> MWHYTSINNDTRVALDPKPNQIRTITKPNTVPQLGTDYLYTFNSQRRSHTLRLLGPFQYFNFSETDRGHPLFRLPLKYPSKAIPADELIDNLHSWMRSVHLLHVRSEDNTLRYNWMLGVYARSTNYTTPVGQLVVNAPAILNYSNPQDAFNSVFVALGIDYIDIPITNSNIFDDSSTPYNVRIWHAPTMTEVNHILALMRKSTLVSTHSSWHWNVLHTFHYRSESDMIDHFAAKILEDWRQKEKLDKGALVEADRVIQRLIPLSSSTYVQRLAAIGALYPNEFTENVLDLSRLSTALLQLSDTYYQHANDQLRRLYRRMYNDSRTLYMTQRHQELLLAQITADPNILLYPYTYIFTTIPTSMNYISNTGQGRIKHSLTVTGATEHDTVADIVLGQTGEDVITISMVEPMSIAVEDMYGYVLDTPTRDIWPADEQIEQKGDAVALYDTKTSRALGMFNNTVRIDDLLSPLLSLVYRTYIKGDTMTMTQGSLDHLTLCAAVDSDITFVGNRMIAPLPEGYIPKPMHRNNSTMKMLSLYVALKKLENFATNSYLMAPDTSIILLGAEREPAVNILRRFNRNVSNVRIIGMGDRAVEPNIRVRVPFPIDKNISADFIICDINSYEDQSFESMFSETISVVTTCASAATRALVKINHPSEYMINSVIERLSQLGGVFYHTALLKTASQNPYSYETYIYITPIAAAVRFPFYSNSAMINRYMTAVADDEMPIIPSIHTVIKGHSNTYSPGLFCGCVDVQSAPLALSQLKSYCSEATTWRVDSDDNLVNIIARIDPARIALEFRTRSNTSAYHEYQRYVPNGLGFKVRKTREFRYMHREVTFIHKLMMYALIREQISLTENMTQVVSIGGRNLADISVVPLNMKYVVIDPATRIETLTQEKKNIEVQSRPFQFDAANMDLENNSIYLFIAVIMNEPNGAATPARMQMDKIRNVATAMLTRTNCVAYISFYEAGIITRLDQSTAHKTIRVEEGRLKVANYVPVDTLVEADVTLMLRDIGITHEIIRPSTPELIDACSNYGIRLGSTGGAVLDVFNHYSPVIKLVRS;>MHSTNNNSNKRNNEEKHKQPEIDSSANNGEGTSGTRAQTVGDTATEAGVRNETEAGASTRRQTDGTGLSGTNAKIATASSARQADVEKPADVTFTIENVDDVGIMQQKKPPTVVQSRTDVFNEQFANEALHPTTKVIFNGLDVNTEVQPLSDDFKQISDPKGYLTYSVKYEDQFTKKDKLRASEADDRIVGPTVNLFKYGAAVVNIDLNRDFFDTATGIDLTKGIPLVQDLLVPIGVTAGAEQSAEYVSGLLMVLFKVMTDNRLVIVGETTTPMSNTLSTVVNNVLRTTYHNNVGVNPALLRDFTQVNWLNRDITNMLQQAGTKYGLGLTETRLDYVRLVKTIVGHALNIDHFAASVLNINLRALMEANVTADDRIKALQAHSMISTQFHGPNQGALRPELAFDHDHIIRCLMLAAANYPRLEGIIVQINTGYVASANVIRPVSEKRYFPENLEQNQSAARLVSAVKARASEADISSIHLAIAREVSPMFNVHELKKIAESFEDPSSIVVVLEFILFALFFPTEFNRIKGDIQNVLLLFFSRWYPVEYGIFVQRGATYTINAAGEFEFSGRNEKWDQALYLSEHFPALFSDVPLAGANTIIAIMRLFTPQGFLRTDDLAIAANFPRASRNPQTYIPYTNQRGTVTNEFASRFRTIVATLANVVNERAVQDDMQKATRSCTKQWLRHLETQFDNIAVAHTDHLSVVYATMSNFMLNFTNNFSGNHATFKPDQYVITSPEGSYKPIIERQGETVDGLTIIDTSIVWPILCQCTYPLVRQSGKGVDAVSIMEEIVYPDPSTTLSQSLSVAQVLSKLTLPDAFINMILSGGDSVVMRTYQTEADDDLDEGIRMTTYDQYLSHIRERLHITNVPDPIYITGASTPDQIAASVQATHVAVVLYQSGVINGPASTYLRENEVLVVMPDYYDVVSRFANANLQMNNNRYHESVLEIADIFDQADFIQTSDAVRQLRALMPTLSTSQIRHAIERIAQITDVDSTDYGKLTLRFLGTLTRSLKMQNAQIRRIRPDGTVLRYDDQIDIEAFRWSRYFLDELQLRRLSVGLRLITNPRIARRFNGVRIMYLTDDDPDPDFVPDVPEGYVAVQYAHRLFSSSLANKRNRVTYTHPPTGMAYPSPTGRPHVHMTINERAGMSKLVADNIIASVIKSNWVVDILDIEYTAEVMTPSEGYTQHVDAESIMTAPKGKLFHLQFMDGLLRPEPSAFDPPASGEDMRLIYPLQPISVARSMRAIVNHNEVDRPRGAVAPSSYEMDTGTLSRNGDLLYSPVANGQVGIPKLEVDHISFSNVVSMMTANIRTGDDMAVERVNPDDVRAINIRNA[2x];>MLQQPTGGYTTLEQFAFTIRNDGTNATPTQFLQLLSYEATENELVKKTIPTPETHLPSARNVPGNVYIEDAITQALFGISAQNVNAHGYFSRLSALALPNTSARLGLDGVIYNSETINIPFYDPAAVANFAATYAKLGNASTPRYRADMIDIYAHVGLELAGTDAERAAGVMPVKRAKFDSWEGSLISLSRDVVNWKILAFLIDLCSLEGEALRAFKTRNRDVFRMMLFIMSTAVAANVVNRKVTKRVDRVLEYIGVNSMRTAGRTATITYDLSRHEFAAKFLQLTFTRWNAASAMIRSMPDMHTPRTSITPAGENALVRHNRYMTENFKGLSPIALAQKKHEMMLHTHEIHSMDIDGSIKNMVERETVNKMNEIDAMNTAPWTEEFAEVEPTTVYERHQIGTDPEQTQLISQDAAVIVHQASSDVDENEYGNSVSELTIDTQSDSVL[2x]

Viral transcription is highly regulated, as demonstrated biochemically in viruses of the Reoviridae. mRNA transcription in these viruses is activated by external actions, for example, removal of their outer shell in multi-shelled reoviruses and binding of S-adenosyl-L-methionine (SAM) in the single-shelled cytoplasmic polyhedrosis virus (CPV). To reveal the mechanisms of transcriptional regulation of viruses within the Reoviridae family, we determined the cryoEM structures of six CPV/ligand complexes in the presence of magnesium ion: CPV+SAM (i.e., ‘S-CPV’), CPV+SAM+4 nucleoside triphosphates (NTPs) (i.e., transcribing, or ‘t-CPV’), CPV+SAM+GTP+ATP (i.e., ‘SGA-CPV’), CPV+SAM +GTP (i.e., ‘SG-CPV’), CPV+GTP (i.e., ‘G-CPV’), and CPV+ATP (i.e., ‘A-CPV’) at resolutions ranging from 2.9 to 3.1 Å. Like the atomic model of unliganded CPV, the atomic models of these liganded CPV all contain two conformers of the capsid shell proteins (CSP-A and CSP-B), two conformers of the large protrusion proteins (LPP-3 and LPP-5), and one conformer of TP in each asymmetrical unit. We discovered that the large sub-domain of guanylyltransferase (GTase) domain of CPV turret protein (TP) also has an ATP-binding site and is likely an ATPase that mediates the activation process of viral RNA transcription and capping.

In order to find out how SAM does this, we obtained a structure of t-CPV at 3.0 Å resolution, that is, virions incubated with SAM, 4 NTPs, and Mg2+. In contrast to that of S-CPV, the cryoEM image of t-CPV shows string-like densities emanating from the viral particles, which we attribute to newly synthesized mRNA molecules in the process of release from the actively transcribing virions. In t-CPV and SGA-CPV, two SAM molecules bind to the MT-1 and MT-2 domains, one Mg2+-GTP to the GTase site and one ATP to the putative ATPase site. All domains of TP undergo global outwards movements (∼9 Å), while only the MT-1 domain and the large sub-domain of GTase domain of TP exhibit local conformation changes. CSP-A not only rotates outwards (up to 9 Å) around a pivot point near the twofold axis (global domain movements indicated by dashed ellipses in Figure 3D and Video 5), but it also changes conformation in its apical domain (dotted ellipse in Figure 3D). CSP-B also undergoes similar but less obvious changes than CSP-A. These structural changes in CSP molecules result in an enlarged, yet stable capsid of the transcribing CPV. The density of the unexpected ligand is as strong as that of the GTP bound to the GTase site and the surrounding amino acid residues, and it fits very well with the atomic model of an ATP molecule, suggesting that the large sub-domain of GTase domain of TP could also be a viral ATP-binding site. Compared to that of G-CPV, the opening (or ‘gate’) leading to the GTase site and coupled to the putative mRNA releasing hole is widened from 13 to 15 Å in t-CPV, likely to accommodate nascent mRNA.>[2x]TPLGPKWPEPVFGRLASPGFPGEYANDQERRWTLTAPPGYRLRLYFT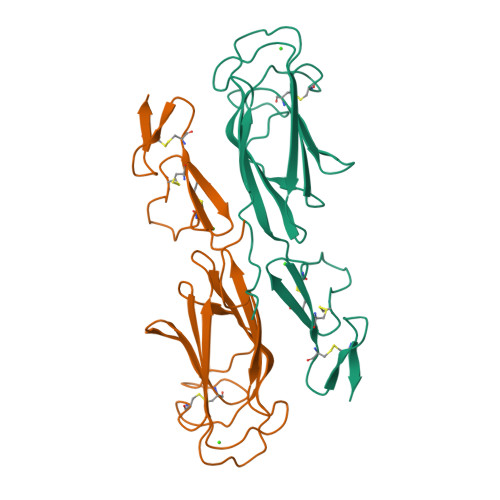HFDLELSHLCEYDFVKLSSGAKVLATLCGQESTDTERAPGKDTFYSLGSSLDITFRSDYSNEKPFTGFEAFYAAEDIDECQVAPGEAPTCDHHCHNHLGGFYCSCRAGYVLHRNKRTCSEQSL> AVRENALLSSSLWVNVALAGIAILVFV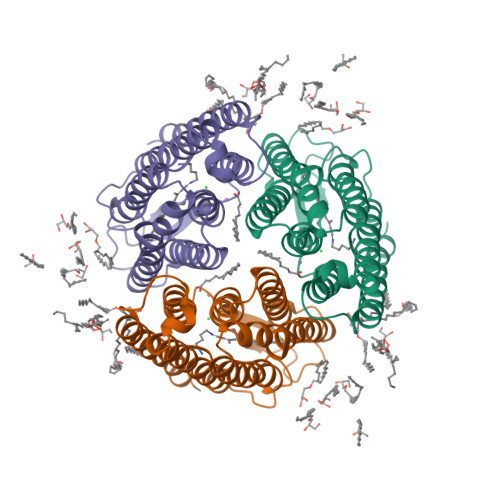YMGRTIRPGRPRLIWGATLMIPLVSISSYLGLLSGLTVGMIEMPAGHALAGEMVRSQWGRYLTWALSTPMILLALGLLADVDLGSLFTVIAADIGMCVTGLAAAMTTSALLFRWAFYAISCAFFVVVLSALVTDWAASASSAGTAEIFDTLRVLTVVLWLGYPIVWAVGVEGLALVQSVGATSWAYSVLDVFAKYVFAFILLRWVANNERTVAVAGQTLGTMSSDD> MSNITIYHNPACGTSRNTLEMIRNSGTEPTIILYLENPPSRDELVKLIADMGISVRALLAKNVEPYEQLGLAEDKFTDDQLIDFMLQHPILINRPIVVTPLGTRLCRPSEVVL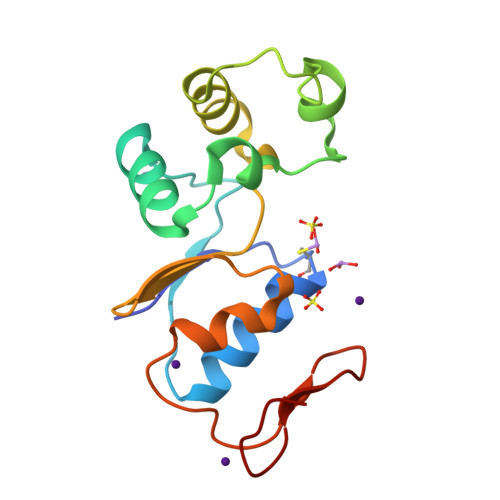DILQDAQKGAFTKEDGEKVVDEAGKRL COENZYME F420-4 | C39 H50 N7 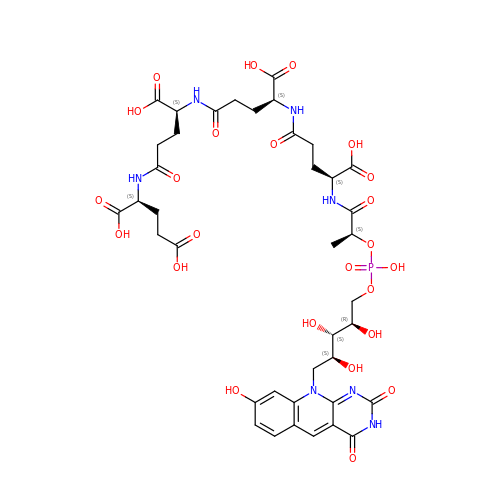O24 P | HYGZFZXLFYAPGM-DKJXVAHLSA-N> GIHHVSIKDVLSKYVQLLPNGSSEFRVVKEKDGSSEILTENQVTFDTKTTSEGLVEVTAKFSPNYSLEDGARYVLKFTVTSSQEALDAIAGDKKLEAGDAEGSDVNKLYSNKGASVTYSYGIGNSQTKTKEYSDNPTFKPSDPLTVPVEVEWQGVTGARTVITADQPSNVELKLVQKNKNGGSDNQDYRKTNVNVSKNVSNETRNFEKVAKGYQYDLIAPDVPAFTKEIKNVGTESNPSFKVIYKQLPSLTIKKVLEAENNLNKEFRIKVKLTSPDSKPLNGTFGEITVVNGEAEIRVEKRKRWRGILSYLPRGTHYKVEEEAASTNGYHVTYENQEGDL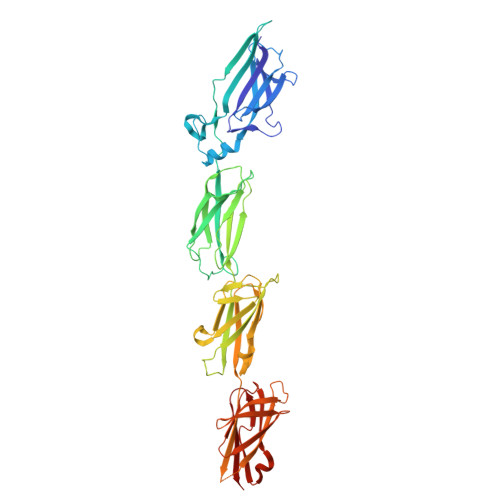NKDETSTVTNHKLPSLSVTKKVTGVFANLLKSFKITINIRDAQNSPLNGTYTATVNNKRTPLQFTNGRASIDLNKDQTIKIDGLPLDSHYTVEEETNSSRGYQVSYENQEGKLDGDKSATVTNNKN> KETAAAKFERQHMDSSTSAASSSNYCNQMMKS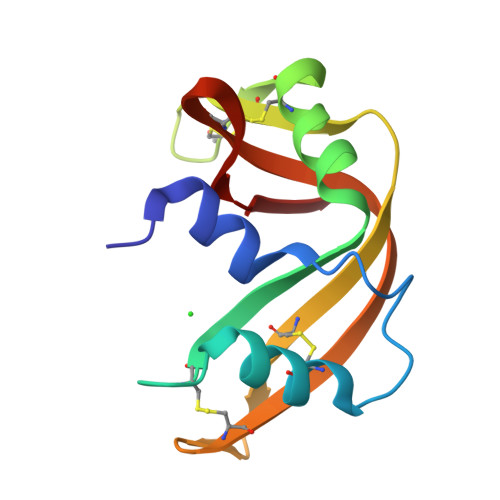RNLTKDRCKPVNTFVHESLADVQAVCSQKNVACKNGQTNCYQSYSTMSITDCRETGSSKYPNCAYKTTQANKHIIVACEGNPYVPVHFAASV2-{(2S)-1-[(4-ethoxyphenyl)methyl]-4-[(2E)-3-(4-methoxyphenyl)prop-2-en-1-yl]piperazin-2-yl}ethan-1-ol 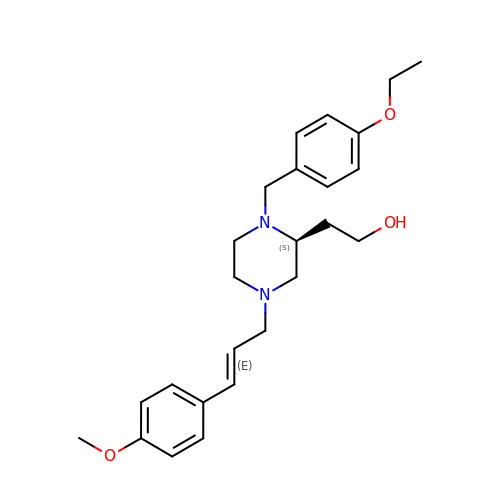| C25 H34 N2 O3 | MBXADFLSFSJJOZ-OIUIXCLQSA-N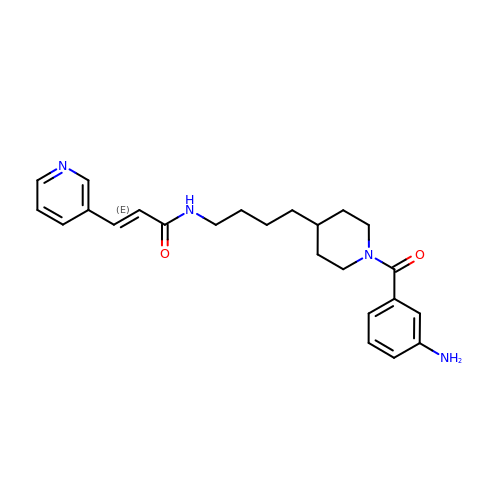(2E)-N-{4-[1-(3-aminobenzene-1-carbonyl)piperidin-4-yl]butyl}-3-(pyridin-3-yl)prop-2-enamide | C24 H30 N4 O2 | JLAJCUOAEWKJJS-MDZDMXLPSA-N(2R,3R)-2-hexyl-3-hydroxytridecanoic acid | C19 H38 O3 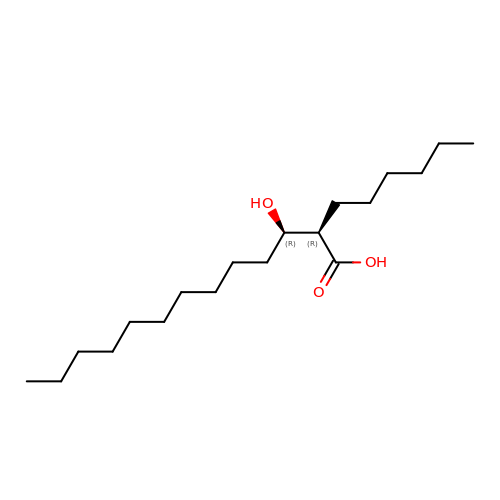| OYDUHHOWTJLUGL-QZTJIDSGSA-N> STDNAETGVIEAGNTDTDFSGELAAPGSNHTNVKFLFDRSRLLNVIKVLEKDAVFPRPFPTQEGAQQDDGYFCLLTPRPTVASRPATRFGLYANPSGSGVLANTSLDFNFYSLACFTYFRSDLEVTVVSLEPDLEFAVGWFPSGSEYQASSFVYDQLHVPFHFTGRTPRAFASKGGKVSFVLPWNSVSSVLPVRWGGASKLSSATRGLPAHADWGTIYAFVPR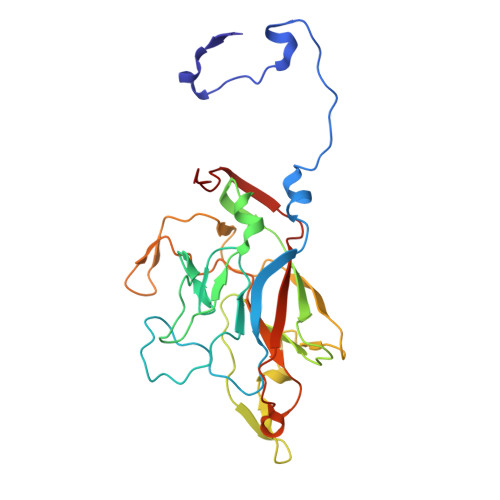PNEKKSTAVKHVAVYIRYKNARAWCPSMLPFRSYK>MHHHHHHSAGENLYFQGKEWQENKSWNAHFTEHKSQGVVVLWNENKQQGFTNNLKRANQAFLPASTFKIPNSLIALDLGVVKDEHQVFKWDGQTRDIATW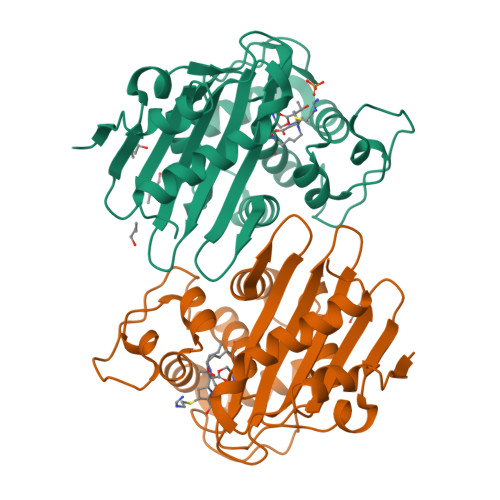NRDHNLITAMKYSVVPVYQEFARQIGEARMSKMLHAFDYGNEDISGNVDSFWLDGGIRISATEQISFLRKLYHNKLHVSERSQRIVKQAMLTEANGDYIIRAKTGYSTRIEPKIGWWVGWVELDDNVWFFAMNMDMPTSDGLGLRQAITKEVLKQEKIIP[2x]>MIINNLKLIREKKKISQSELAALLEVSRQTINGIEKNKYNPSLQLALKIAYYLNCPLE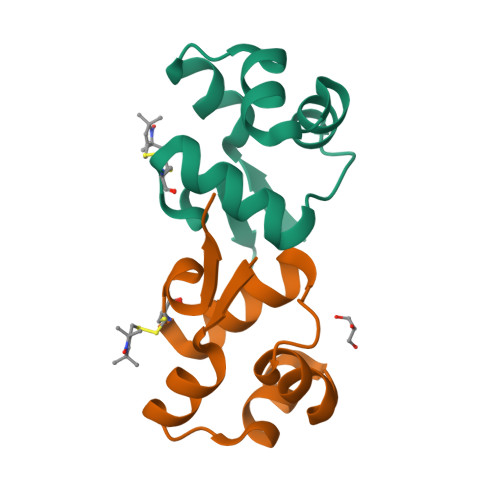DIFQWQPE[2x]> GAMAGKSS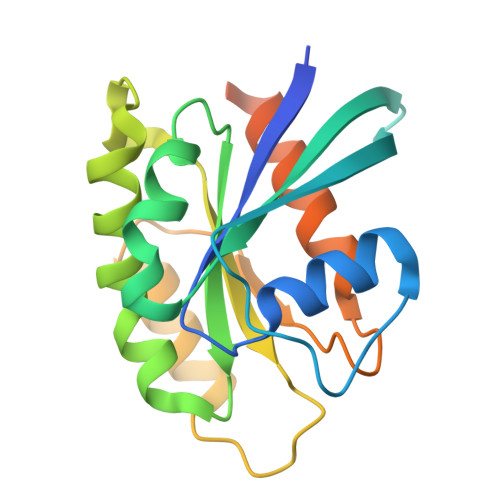LFKVILLGDGGVGKSSLMNRYVTNKFDTQLFHTIGVEFLNKDLEVDGHFVTMQIWDTAGLERFRSLRTPFYRGSDCCLLTFSVDDSQSFQNLSNWKKEFIYYADVKEPESFPFVILGNKIDISERQVSTEEAQAWCRDNGDYPYFETSAKDATNVAAAFEEAVRRVLATEDRSDHLIQTDTVNLHRKPKPSSSCC>SPSSGLGSITDLLNNILSVANQIIYNSAVALPLQLDT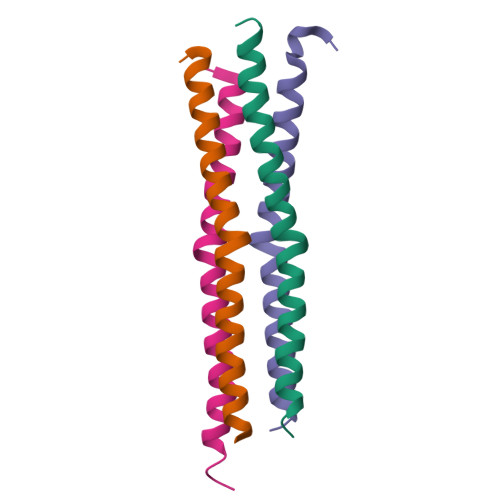LESTLLTAIKSLQTSDKLEQNCSWSAAL[4x]> AFTDVPALNYPATPPP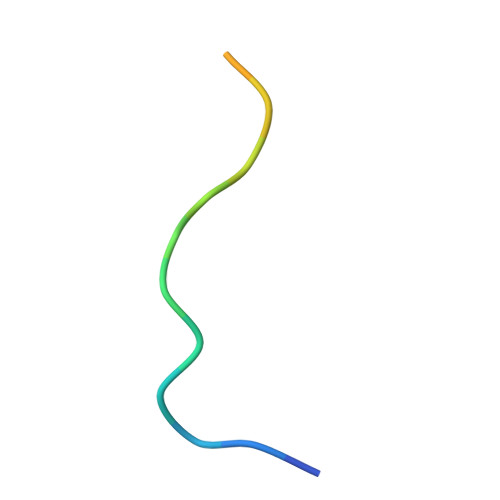H> SLGTSEAAPPPFARVAPALFIGNARAAGATELLVRAGITLCVNVSRQQPGPRAPGVAELRVPVFDDPAEDLLTHLEPTCAAMEAAVRDGGSCLVYCKNGRSRSAAVCTAYLMRHRGHSLDRAFQMVKSARPVAEPNLGFWAQLQKYEQ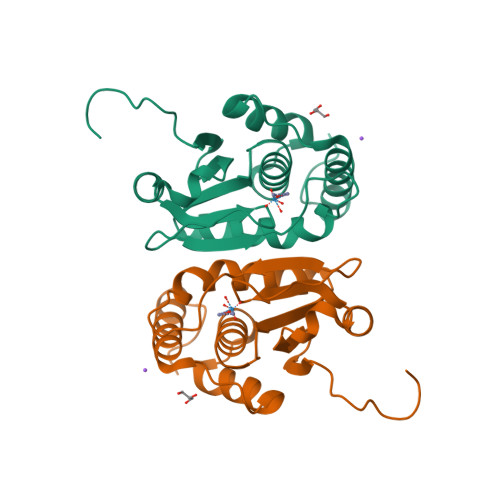TLQAQAILPREPIDPE>[4x]SHMRVLVCGGAGYIGSHFVRALLRDTNHSVVIVDSLVGTHGKSDHVETRENVARKLQQSDGPKPPWADRYAALEVGDVRNE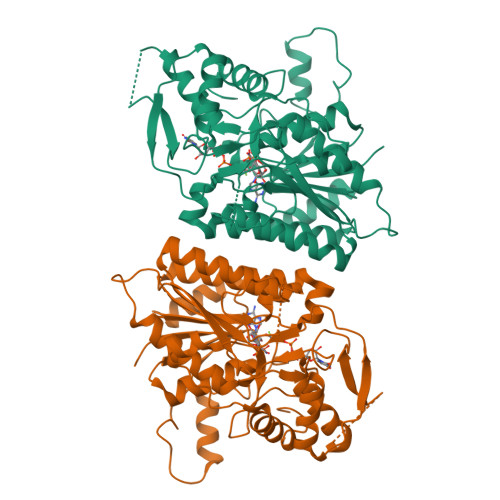DFLNGVFTRHGPIDAVVHMCAFLAVGESVRDPLKYYDNNVVGILRLLQAMLLHKCDKIIFSSSAAIFGNPTMGSVSTNAEPIDINAKKSPESPYGESKLIAERMIRDCAEAYGIKGICLRYFNACGAHEDGDIGEHYQGSTHLIPIILGRVMSDIAPDQRLTIHEDASTDKRMPIFGTDYPTPDGTCVRDYVHVCDLASAHILALDYVEKLGPNDKSKYFSVFNLGTSRGYSVREVIEVARKTTGHPIPVRECGRREGDPAYLVAASDKAREVLGWKPKYDTLEAIMETSWKFQRTHPNGYASQENGTPGGRTTKL Maintaining the optimal nucleotide balance required for normal cell proliferation is controlled by 5′-nucleotidases amongst other processes. These enzymes catalyze the dephosphorylation of ribo- and deoxyribonucleoside monophosphates to their corresponding nucleosides, and also exhibit, in certain cases phosphotransferase activity. All structures adopt a tetrameric assembly displaying a cross-like shape, in agreement with the quaternary solution structure. Each subunit consists of four domains: an “N-Terminal Regulatory Domain” (NTRD, M1 to K59), an “OD” (D60 to T143), a HAD-like Catalytic Domain (CD, F144 to K270 and K371 to Q444) and a C2 cap domain13 (K271 to N370).

Structure- and functional analyses revealed the essential role of NTRDs in the catalytic mechanism of PfISN1. Moreover, deletion of the NTRDs (PfISN1-∆N59) inactivates the enzyme at pH 8, while at pH 5 there is a sixfold drop in activity. Indeed, the structure of PfISN1-∆N59 co-crystallized with IMP shows that when lacking NTRDs, SegmentD394-F407 cannot be stabilized (not well defined in the electron density), and consequently the enzyme is no longer able to accommodate the substrate correctly (IMP not observed in the crystal structure). We demonstrated that when lacking NTRDs as in PfISN1-ΔN59 the activity is highly compromised. This is likely due to its incapacity to stabilize SegmentD394-F407 containing the ubiquitous HAD family motif IV, which is mandatory for coordinating IMP-Mg2+.

>[2x]DSLIMFLVEIFRSLFVSNCIDKNIDNVLLSIEEMFIDHYYNPQHSRLKYLIDDVGIFFTKLPITKAFHTYNKKYRITKRLYAPPTFNEVRHILNLAQILSLEEGLDLLTFDADETLYPDGHDFNDEVLASYISCLLKKMNIAIVTAASYNNDAEKYQKRLENLLKYFSKHNIKDGSYKNFYVMGGESNYLFKCNEEATLYSVPENEWRHYKKFVDYDTVQEILNISEKCLEKVIKDFGLCAQIQRKEKSIGLVPNKIPSLNIKNEQKNYMIKYEVLEEAVIRIKKEIIKNKITAPYCAFNGGQDLWVDVGNKAEGLLILQKLLKIQKKKCCHIGDQFLHSGNDFPTRFCSLTLWVSNPQETKACLKSIMHLNIKSFIPEVLYENQ> GSSGAFEDRDPTQFEERHLKFLQQLGKGNFGSVEMCRYDPLQDNTGEVVAVKKLQHSTEEHLRDFEREIEILKSLQHDNIVKYKGVCYSAGRRNLKLIMEYLPYGSLRDYLQKHKERIDHIKLLQYTSQICKGMEYLGTKRYIHRDLATRNILVENENRVKIGDFGLTKVLPQDKEYYKVKEPGESPIFWYAPESLTESKFSVASDVWSFGVVLYELFTYIEKSKSPPAEF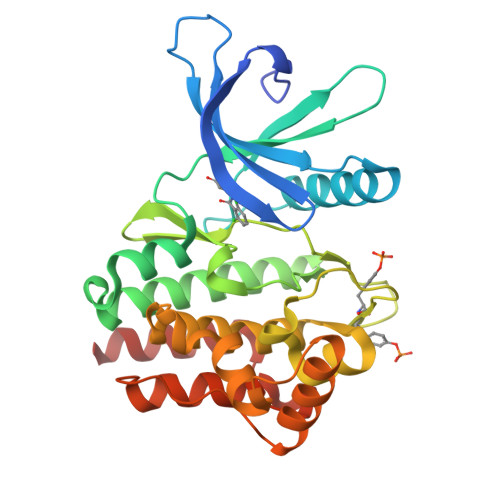MRMIGNDKQGQMIVFHLIELLKNNGRLPRPDGCPDEIYMIMTECWNNNVNQRPSFRDLALRVDQIRDNMAG> SPNSQYLKTRILDIYTPEQRAGIEKSEDWRQFSRRMDTHFPKLMNELDSVYGNNEALLPMLEMLLAQAWQSYSQRNSSLKDIDIARENNPDWILSNKQVGGVCYVDLFAGDLKGLKDKIPYFQELGLTYLHLMPLFKCPEGKSDGGYAVSSYRDVNPALGTIGDLREVIAALHEAGISAVVDFIFNHTSNEHEWAQRCAAGDPLFDNFYYIFPDRRMPDQYDRTLREIFPDQHPGGFSQLEDGRWVWTTFNSFQWDLNYSNPWVFRAMAGEMLFLANLGVDILRMDAVPCIWKQMGTSCENLPQAHALIRAFNAVMRIAAPAVFFKSEAIVHPDQVVQYIGQDECQIGYNPLQMALLWNTLATREVNLLH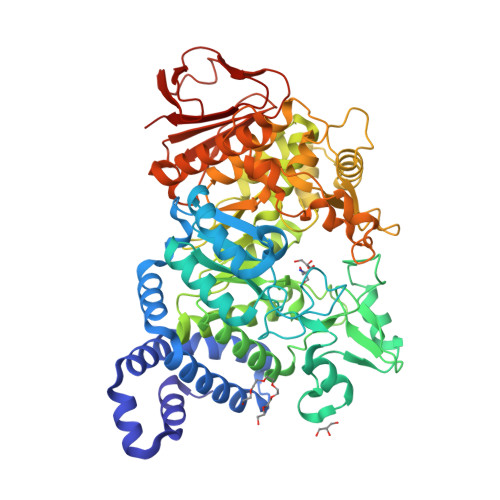QALTYRHNLPEHTAWVNYVRSHDDIGWTFADEDAAYLGISGYDHRQFLNRFFVNRFDGSFARGVPFQYNPSTGDCRVSGTAAALVGLAQDDPHAVDRIKLLYSIALSTGGLPLIYLGDEVGTLNDDDWSQDSNKSDDSRWAHRPRYNEALYAQRNDPSTAAGQIYQDLRHMIAVRQSNPRFDGGRLVTFNTNNKHIIGYIRNNALLAFGNFSEYPQTVTAHTLQAMPFKAHDLIGGKTVSLNQDLTLQPYQVMWLEIA N-HYDROXYMETHYL-N-(2-METHOXYETHYL)-DAUNOMYCIN | C31 H39 N O12 | 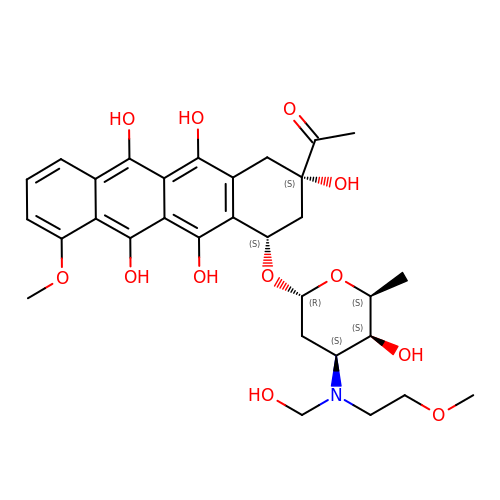IURHBLXSEHXXFF-XGGCRALDSA-N>[4x]MNRESFAAGERLVSPAYVRQGCEARRSHEHLIRLLLEKGKCPENGWDESTLELFLHELAIMDSNNFLGNCGVGEREGRVASALVARRHYRFIHGIGRSGDISAVQPKAAGSSLLNKITNSLVLDIIKLAGVHTVANCFVVPMATGMSLTLCFLTLRHKRPKAKYIIWPRIDQ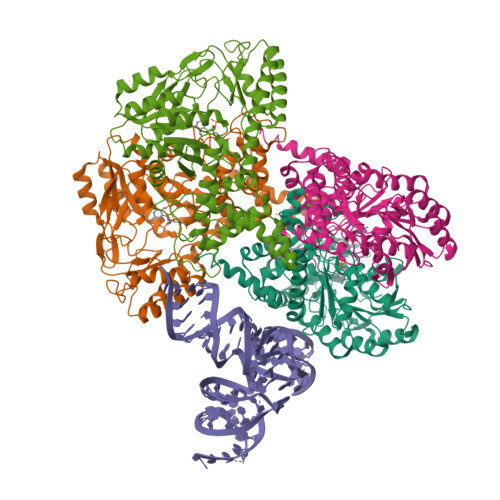KSCFKSMITAGFEPVVIENVLEGDELRTDLKAVEAKVQELGPDCILCIHSTTSCFAPRVPDRLEELAVICANYDIPHIVNNAYGVQSSKCMHLIQQGARVGRIDAFVQSLDKNFMVPVGGAIIAGFNDSFIQEISKMYPGRASASPSLDVLISLLSLGSNGYKKLLKERKEMFSYLSNQIKKLSEAYNERLLHTPHNPISLAMTLKTLDEHRDKAVTQLGSMLFTRQVSGARVVPLGSMQTVSGYTFRGFMSHTNNYPCAYLNAASAIGMKMQDVDLFIKRLDRCLKAVRKERSKESDDNYDKTEDVDIEEMALKLDNVLLDTYQDASS> MAFEALTGINGDLITRSWSASKQAYLTERYHKEEAGAVVIFAFQPSFSEKDFFDPDNKSSFGEIKLNRVQFPCMRKIGKGDVATVNEAFLKNLEAIIDPRTSFQASVEMAVRSRKQIVFTGHSSGGATAILATVWYLEKYFIRNPNVYLEPRCVTFGAPLVGDSIFSHALGREKWSRFFVNFVSRFDIVPRIMLARKASVEETLPHVLAQLDPRKSSVQESEQRITEFYTRVMRDTSTVANQAVCELTGSAEAFLETLSSFLELSPYRPAGTFVFSTEKRLVAVNNSDAILQMLFYTSQASDEQEWSLIPFRSIRDHHSYEELVQSMGKKLFNHLDGENSIESTLNDLGVSTRGRQYVQAALEEEKKRVENQKKIIQVIEQERFLKKLAWIEDEYKPKCQAHKNGYYDSFKVSNEENDFKANVKRAELAGVFDEVLGLMKKCQLPDEFEGDIDWIKLATRYRRLVEPLDIANYHRHLKNEDTGPYMKRGRPTRYIYAQRGYEHYILKPNGMIAEDVFWNKVNGLNLGLQLEEIQETLKNSGSECGSCFWAEVEELKGKPYEEVEVRVKTLEGMLGEWITDGEVDDKEIFLEGSTFRKWWITLPKNHKSHSPLRDYMMDEITDT;> MESSSSLKGSALGKLVVTSGLLHSSWSKILEIHNPPYSNHDPGLQVSKKKKDSGLEFQIHREEKFTLVVFSAPPICRSSSSDSTLLHVKDKENPFPFLCSENNPSFSLHTPAFNLFTSASTSLTYLKSELLQTLKSEKPVIITGAAL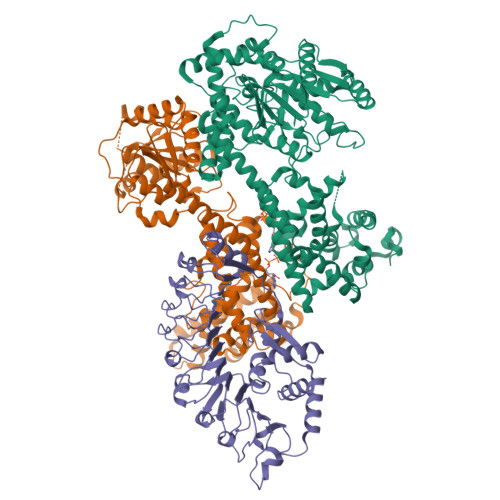GGSVASLYTLWLLETIEPTLKRPLCITFGSPLIGDASLQQILENSVRNSCFLHVVSAQTRIKMDFFKPFGTFLICFDSGCVCIEDHVAVTELLNGVHDSGLVDYSQVLNRLDQSMLSLADSRLIPEDVIKGIEKRAEMKNLRFDMMFKKLNDMKISMAYIEWYKKKCKEVKIGYYDRFKTQLAFPSKEFDINIKNHHKSELNRFWKSVVEEVERRPQSDASILKRRFLFSGNNYRRMIEPLDIAEYYLEGRKEYRTTGRSHHYVMLEKWFGMESILIEKERCKKRDLSDLLTFDSCFWAEVEDSLIVINQLNTTVGMRDDVREVLTRKLVEFEGYVWEIITKREVSPEIFLEESSFMKWWKEYKKIKGFNSSYLTEFMNTRKYESYGKSQ;> MNSNSIQSFDALPHNLRECFLDMASFLEDQRIIASTIIDLWSASYGKEGMNNLQDLASRNLLKLLPIGRNEYEDGFYNELLVKQDNVLREFAINQCLKESSSIFERKRLNLEIQDNKFPNWCLNPKQPIVINASLFSISTDDSFASSWFEMDCPNVEALVLNISSSNYALPNFIATMKELKVVIIINHGLEPAKLTNLSCLSSLPNLKRIRFEKVSISLLDIPKLGLKSLEKLSLWFCHVVDALNELEDVSETLQSLQEIEIDYCYNLDELPYWISQVVSLKKLSVTNCNKLCRVIEAIGDLRDLETLRLSSCASLLELPETIDRLDNLRFLDVSGGFQLKNLPLEIGKLKKLEKISMKDCYRCELPDSVKNLENLEVKCDEDTAFLWKILKPEMKNLTITEEKTEHNLNLLQLF> QETEDPACCSPIVPRNEWKALASECAQHLSLPLRYVVVSHTAGSSCNTPASCQQQARNVQHYHMKTLGWCDVGYNFLIGEDGLVYEGRGWNFTGAHSGHL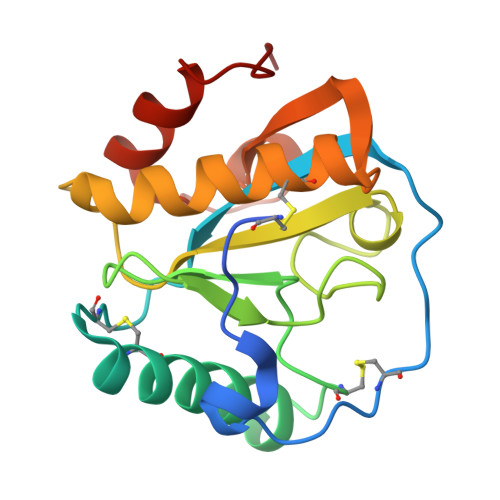WNPMSIGISFMGNYMDRVPTPQAIRAAQGLLACGVAQGALRSNYVLKGHRDVQRTLSPGNQLYHLIQNWPHYRSP> GSPGIHMAWRSVGANNEDLIRQLKDHGVIASDAV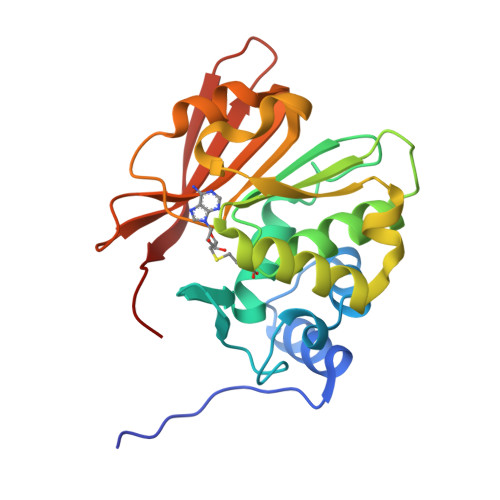AQAMKETDRKHYSPRNPYMDAPQPIGGGVTISAPHMHAFALEYLRDHLKPGARILDVGSGSGYLTACFYRYIKAKGVDADTRIVGIEHQAELVRRSKANLNTDDRSMLDSGQLLIVEGDGRKGYPPNAPYNAIHVGAAAPDTPTELINQLASGGRLIVPVGPDGGSQYMQQYDKDANGKVEMTRLMGVMYVPL> EMVDNLRGKSGQGYYVEMTVGSPPQTLNILVDTGSSNFAVGAAPHPFLHRYYQRQLSSTYRDLRKGVYVPYTQGKWEGELGTDLVSIPHGPNVTVRANIAAITESDKFFINGSNWEGILGLAYAEIARPDDSLEPFFDSLVKQTHVPNLFSLQLCGAGFPL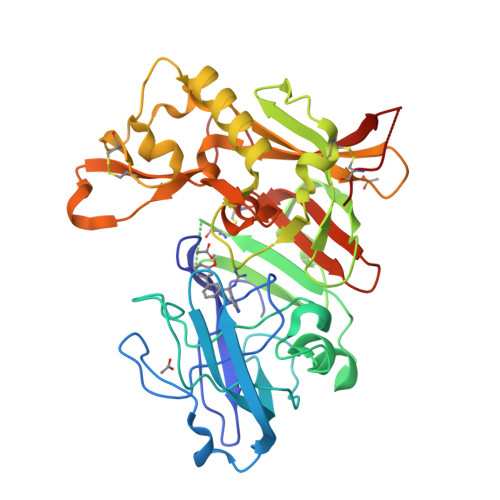NQSEVLASVGGSMIIGGIDHSLYTGSLWYTPIRREWYYEVIIVRVEINGQDLKMDCKEYNYDKSIVDSGTTNLRLPKKVFEAAVKSIKAASSTEKFPDGFWLGEQLVCWQAGTTPWNIFPVISLYLMGEVTNQSFRITILPQQYLRPVEDVATSQDDCYKFAISQSSTGTVMGAVIMEGFYVVFDRARKRIGFAVSACHVHDEFRTAAVEGPFVTLDMEDCGY> MSDNRRRRREEDDSDSENELPPSSPQQHFRGGMNPVSSPIGSPDMINPEGDDNEVDDVPDIDEVEEQMNEVDLMDDNMYEDYAADHNRDRYDPDQVDDREQQELSLSERRRIDAQLNERDRLLRNVAYIDDEDEEQEGAAQLDEMGLPVQRRRRRRQYEDLENSDDDLLSDMDIDPLREELTLESLSNVKANSYSEWITQPNVSRTIARELKSFLLEYTDETGRSVYGARIRTLGEMNSESLEVNYRHLAESKAILALFLAKCPEEMLKIFDLVAMEATELHYPDYARIHSEIHVRISDFPTIYSLRELRESNLSSLVRVTGVVTRRTGVFPQLKYVKFNCLKCGSILGPFFQDSNEEIRISFCTNCKSKGPFRVNGEKTVYRNYQRVTLQEAPGTVPPGRLPRHREVILLADLVDVSKPGEEVEVTGIYKNNYDGNLNAKNGFPVFATIIEANSIKRREGNTANEGEEGLDVFSWTEEEEREFRKISRDRGIIDKIISSMAPSIYGHRDIKTAVACSLFGGVPKNVNGKHSIRGDINVLLLGDPGTAKSQILKYVEKTAHRAVFATGQGASAVGLTASVRKDPITKEWTLEGGALVLADKGVCLIDEFDKMNDQDRTSIHEAMEQQSISISKAGIVTTLQARCSIIAAANPNGGRYNSTLPLAQNVSLTEPILSRFDILCVVRDLVDEEADERLATFVVDSHVRSHPENDEDREGEELKNNGESAIEQGEDEINEQLNARQRRLQRQRKKEEEISPIPQELLMKYIHYARTKIYPKLHQMDMDKVSRVYADLRRESISTGSFPITVRHLESILRIAESFAKMRLSEFVSSYDLDRAIKVVVDSFVDAQKVSVRRQLRRSFAIYTLGH;> MDYKDHDGDYKDHDIDYKDDDDKGGRMEGSTGFDGDATTFFAPDAVFGDRVRRFQEFLDTFTSYRDSVRSIQVYNSNNAANYNDDQDDADERDLLGDDDGDDLEKEKKAASSTSLNILPHRIIISLDDLREFDRSFWSGILVEPAYFIPPAEKALTDLADSMDDVPHPNASAVSSRHPWKLSFKGSFGAHALSPRTLTAQHLNKLVSVEGIVTKTSLVRPKLIRSVHYAAKTGRFHYRDYTDATTTLTTRIPTPAIYPTEDTEGNKLTTEYGYSTFIDHQRITVQEMPEMAPAGQLPRSIDVILDDDLVDKTKPGDRVNVVGVFKSLGAGGMNQSNSNTLIGFKTLILGNTVYPLHARSTGVAARQMLTDFDIRNINKLSKKKDIFDI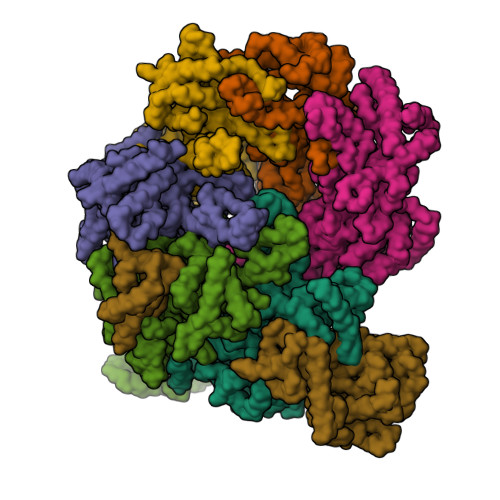LSQSLAPSIYGHDHIKKAILLMLMGGVEKNLENGSHLRGDINILMVGDPSTAKSQLLRFVLNTASLAIATTGRGSSGVGLTAAVTTDRETGERRLEAGAMVLADRGVVCIDEFDKMTDVDRVAIHEVMEQQTVTIAKAGIHTTLNARCSVIAAANPVFGQYDVNRDPHQNIALPDSLLSRFDLLFVVTDDINEIRDRSISEHVLRTHRYLPPGYLEGEPVRERLNLSLAVGEDADINPEEHSNSGAGVENEGEDDEDHVFEKFNPLLQAGAKLAKNKGNYNGTEIPKLVTIPFLRKYVQYAKERVIPQLTQEAINVIVKNYTDLRNDDNTKKSPITARTLETLIRLATAHAKVRLSKTVNKVDAKVAANLLRFALLGEDIGNDIDEEESEYEEALSKRSPQKSPKKRQRVRQPASNSGSPIKSTPRRSTASSVNATPSSARRILRFQDDEQNAGEDDNDIMSPLPADEEAELQRRLQLGLRVSPRRREHLHAPEEGSSGPLTEVGTPRLPNVSSAGQDDEQQQSVISFDNVEPGTISTGRLSLISGIIARLMQTEIFEEESYPVASLFERINEELPEEEKFSAQEYLAGLKIMSDRNNLMVADDKVWRV;> MSQQSSSPTKEDNNSSSPVVPNPDSVPPQLSSPALFYSSSSSQGDIYGRNNSQNLSQGEGNIRAAIGSSPLNFPSSSQRQNSDVFQSQGRQGRIRSSASASGRSRYHSDLRSDRALPTSSSSLGRNGQNRVHMRRNDIHTSDLSSPRRIVDFDTRSGVNTLDTSSSSAPPSEASEPLRIIWGTNVSIQECTTNFRNFLMSFKYKFRKILDEREEFINNTTDEELYYIKQLNEMRELGTSNLNLDARNLLAYKQTEDLYHQLLNYPQEVISIMDQTIKDCMVSLIVDNNLDYDLDEIETKFYKVRPYNVGSCKGMRELNPNDIDKLINLKGLVLRSTPVIPDMKVAFFKCNVCDHTMAVEIDRGVIQEPARCERIDCNEPNSMSLIHNRCSFADKQVIKLQETPDFVPDGQTPHSISLCVYDELVDSCRAGDRIEVTGTFRSIPIRANSRQRVLKSLYKTYVDVVHVKKVSDKRLDVDTSTIEQELMQNKVDHNEVEEVRQITDQDLAKIREVAAREDLYSLLARSIAPSIYELEDVKKGILLQLFGGTNKTFTKGGRYRGDINILLCGDPSTSKSQILQYVHKITPRGVYTSGKGSSAVGLTAYITRDVDTKQLVLESGALVLSDGGVCCIDEFDKMSDSTRSVLHEVMEQQTISIAKAGIITTLNARSSILASANPIGSRYNPNLPVTENIDLPPPLLSRFDLVYLVLDKVDEKNDRELAKHLTNLYLEDKPEHISQDDVLPVEFLTMYISYAKEHIHPIITEAAKTELVRAYVGMRKMGDDSRSDEKRITATTRQLESMIRLAEAHAKMKLKNVVELEDVQEAVRLIRSAIKDYATDPKTGKIDMNLVQTGKSVIQRKLQEDLSREIMNVLKDQASDSMSFNELIKQINEHSQDRVESSDIQEALSRLQQEDKVIVLGEGVRRSVRLNNRV;> MSFDRPEIYSAPVLQGESPNDDDNTEIIKSFKNFILEFRLDSQFIYRDQLRNNILVKNYSLTVNMEHLIGYNEDIYKKLSDEPSDIIPLFETAITQVAKRISILSRAQSANNNDKDPENTSMDTDSLLLNSLPTFQLILNSNANQIPLRDLDSEHVSKIVRLSGIIISTSVLSSRATYLSIMCRNCRHTTSITINNFNSITGNTVSLPRSCLSTIESESSMANESNIGDESTKKNCGPDPYIIIHESSKFIDQQFLKLQEIPELVPVGEMPRNLTMTCDRYLTNKVIPGTRVTIVGIYSIYNSKNGAGSGRSGGGNGGSGVAIRTPYIKILGIQSDVETSSIWNSVTMFTEEEEEEFLQLSRNPKLYEILTNSIAPSIFGNEDIKKAIVCLLMGGSKKILPDGMRLRGDINVLLLGDPGTAKSQLLKFVEKVSPIAVYTSGKGSSAAGLTASVQRDPMTREFYLEGGAMVLADGGVVCIDEFDKMRDEDRVAIHEAMEQQTISIAKAGITTVLNSRTSVLAAANPIYGRYDDLKSPGDNIDFQTTILSRFDMIFIVKDDHNEERDISIANHVINIHTGNANAMQNQQEENGSEISIEKMKRYITYCRLKCAPRLSPQAAEKLSSNFVTIRKQLLINELESTERSSIPITIRQLEAIIRITESLAKLELSPIAQERHVDEAIRLFQASTMDAASQDPIGGLNQASGTSLSEIRRFEQELKRRLPIGWSTSYQTLRREFVDTHRFSQLALDKALYALEKHETIQLRHQGQNIYRSGV;> MSSPFPADTPSSNRPSNSSPPPSSIGAGFGSSSGLDSQIGSRLHFPSSSQPHVSNSQTGPFVNDSTQFSSQRLQTDGSATNDMEGNEPARSFKSRALNHVKKVDDVTGEKVREAFEQFLEDFSVQSTDTGEVEKVYRAQIEFMKIYDLNTIYIDYQHLSMRENGALAMAISEQYYRFLPFLQKGLRRVVRKYAPELLNTSDSLKRSEGDEGQADEDEQQDDDMNGSSLPRDSGSSAAPGNGTSAMATRSITTSTSPEQTERVFQISFFNLPTVHRIRDIRSEKIGSLLSISGTVTRTSEVRPELYKASFTCDMCRAIVDNVEQSFKYTEPTFCPNPSCENRAFWTLNVTRSRFLDWQKVRIQENANEIPTGSMPRTLDVILRGDSVERAKPGDRCKFTGVEIVVPDVTQLGLPGVKPSSTLDTRGISKTTEGLNSGVTGLRSLGVRDLTYKISFLACHVISIGSNIGASSPDANSNNRETELQMAANLQANNVYQDNERDQEVFLNSLSSDEINELKEMVKDEHIYDKLVRSIAPAVFGHEAVKKGILLQMLGGVHKSTVEGIKLRGDINICVVGDPSTSKSQFLKYVVGFAPRSVYTSGKASSAAGLTAAVVRDEEGGDYTIEAGALMLADNGICCIDEFDKMDISDQVAIHEAMEQQTISIAKAGIHATLNARTSILAAANPVGGRYNRKLSLRGNLNMTAPIMSRFDLFFVILDDCNEKIDTELASHIVDLHMKRDEAIEPPFSAEQLRRYIKYARTFKPILTKEARSYLVEKYKELRKDDAQGFSRSSYRITVRQLESMIRLSEAIARANCVDEITPSFIAEAYDLLRQSIIRVDVDDVEMDEEFDNIESQSHAASGNNDDNDDGTGSGVITSEPPADIEEGQSEATARPGTSEKKKTTVTYDKYVSMMNMIVRKIAEVDREGAEELTAVDIVDWYLLQKENDLGSLAEYWEERRLAFKVIKRLVKDRILMEIHGTRHNLRDLENEENENNKTVYVIHPNCEVLDQLEPQDSS;> MSAALPSIQLPVDYNNLFNEITDFLVTFKQDTLSSDATRNENEDENLDAENIEQHLLEKGPKYMAMLQKVANRELNSVIIDLDDILQYQNEKFLQGTQADDLVSAIQQNANHFTELFCRAIDNNMPLPTKEIDYKDDVLDVILNQRRLRNERMLSDRTNEIRSENLMDTTMDPPSSMNDALREVVEDETELFPPNLTRRYFLYFKPLSQNCARRYRKKAISSKPLSVRQIKGDFLGQLITVRGIITRVSDVKPAVEVIAYTCDQCGYEVFQEVNSRTFTPLSECTSEECSQNQTKGQLFMSTRASKFSAFQECKIQELSQQVPVGHIPRSLNIHVNGTLVRSLSPGDIVDVTGIFLPAPYTGFKALKAGLLTETYLEAQFVRQHKKKFASFSLTSDVEERVMELITSGDVYNRLAKSIAPEIYGNLDVKKALLLLLVGGVDKRVGDGMKIRGDINVCLMGDPGVAKSQLLKAICKISPRGVYTTGKGSSGVGLTAAVMKDPVTDEMILEGGALVLADNGICCIDEFDKMDESDRTAIHEVMEQQTISISKAGINTTLNARTSILAAANPLYGRYNPRLSPLDNINLPAALLSRFDILFLMLDIPSRDDDEKLAEHVTYVHMHNKQPDLDFTPVEPSKMREYIAYAKTKRPVMSEAVNDYVVQAYIRLRQDSKREMDSKFSFGQATPRTLLGIIRLSQALAKLRLADMVDIDDVEEALRLVRVSKESLYQETNKSKEDESPTTKIFTIIKKMLQETGKNTLSYENIVKTVRLRGFTMLQLSNCIQEYSYLNVWHLINEGNTLKFVDDGTMDTDQEDSLVSTPKLAPQTTASANVSAQDSDIDLQDA;> MSGTANSRRKEVLRVPVIDLNRVSDEEQLLPVVRAILLQHDTFLLKNYANKAVLDALLAGLTTKDLPDTSQGFDANFTGTLPLEDDVWLEQYIFDTDPQLRFDRKCRNESLCSIYSRLFKLGLFFAQLCVKSVVSSAELQDCISTSHYATKLTRYFNDNGSTHDGADAGATVLPTGDDFQYLFERDYVTFLPTGVLTIFPCAKAIRYKPSTMATTDNSWVSIDEPDCLLFHTGTLLARWSQGMHTTSPLQIDPRANIVSLTIWPPLTTPISSKGEGTIANHLLEQQIKAFPKVAQQYYPRELSILRLQDAMKFVKELFTVCETVLSLNALSRSTGVPPELHVLLPQISSMMKRKIVQDDILKLLTIWSDAYVVELNSRGELTMNLPKRDNLTTLTNKSRTLAFVERAESWYQQVIASKDEIMTDVPAFKINKRRSSSNSKTVLSSKVQTKSSNANALNNSRYLANSKENFMYKEKMPDSQANLMDRLRERERRSAALLSQRQKRYQQFLAMKMTQVFDILFSLTRGQPYTETYLSSLIVDSLQDSNNPIGTKEASEILAGLQGILPMDISVHQVDGGLKVYRWNSLDKNRFSKLLQIHKSKQQD>[2x]MSRPAPLTLIGLGPMGQAMGNALLDRGHGLTVWNRTASRADALVARGAVRAPTVAAAVAANELVVLSLTDYDAMYALLGPAADALAGKVVVNLSSDTPEKTRAGARWIAEHGGTLIAGGVTCPPSGIGSPESSAFYSGPSAAFERHRETLRTLTRTDYRGEDPGLAALWYQIGMV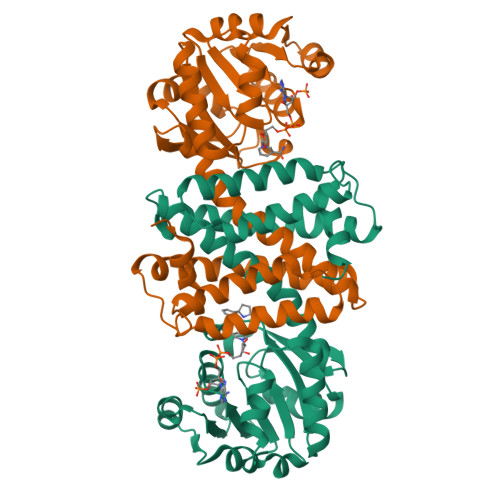MWWNAMLGYLQAVALADANGLKAADILPHASDTVAGLPFFLRFYADRIDTGHHGGDADRLAMGTASVEHILHTMADSGVDTALPEAVVALFRRGEAAGYAENSFSSMVELLKKPS>GASTRDYEIQRERIELGRCIGEGQFGDVHQGIYMSPENPALAVAIKTCKNCTSDSVREKFLQEALTMRQFDHPHIVKLIGVITENPVWIIMELCTLGELRSFLQVRKYSL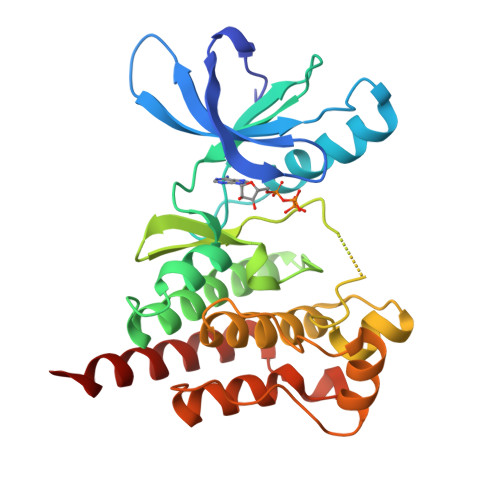DLASLILYAYQLSTALAYLESKRFVHRDIAARNVLVSSNDCVKLGDFGLSRYMEDSTYYKASKGKLPIKWMAPESINFRRFTSASDVWMFGVCMWEILMHGVKPFQGVKNNDVIGRIENGERLPMPPNCPPTLYSLMTKCWAYDPSRRPRFTELKAQLSTILEEEKAQQEE[2x]>MTVQIPKLLFLHGFLQNGKVFSEKSSGIRKLLKKANVQCDYIDAPVLLEKKDLPFEMDDEKWQATLDADVNRAWFYHSEISHELDISEGLKSVVDHIKANGPYDGIVGLSQGAALSSIITNKISELVPDHP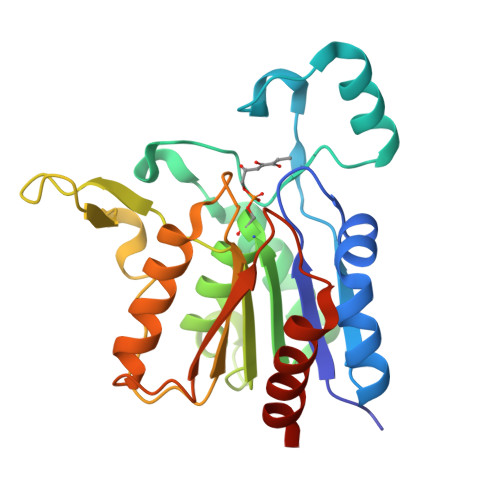QFKVSVVISGYSFTEPDPEHPGELRITEKFRDSFAVKPDMKTKMIFIYGASDQAVPSVRSKYLYDIYLKAQNGNKEKVLAYEHPGGHMVPNKKDIIRPIVEQITSSLQEASE[2x]>GSGSMISIFIAEDQQMLLGALGSLLNLEDDMEVVGKGTTGQDAVDFVKKRQPDVCIMDIEMPGKTGLEAAEELKDTGCKIIILTTFARPGYFQRAIKAGVKGYLLKDSPSEELANAIRSVMNGKRIYAPELMEDLYS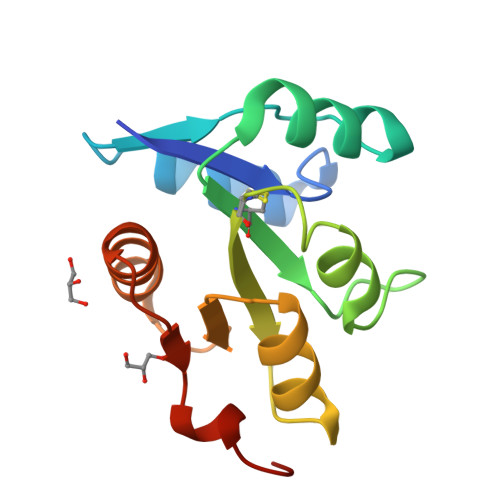EA[2x]> AEVAPGDVAIDGQGHVARPLTDAPGDPVEGRRLMTDRSVGNCIACHEVTEMADAQFPGTVGPSLDGVAARYPEAMIRGILVNSKNVFPETVMPAYYRVEGFNRPGIAFTSKPIE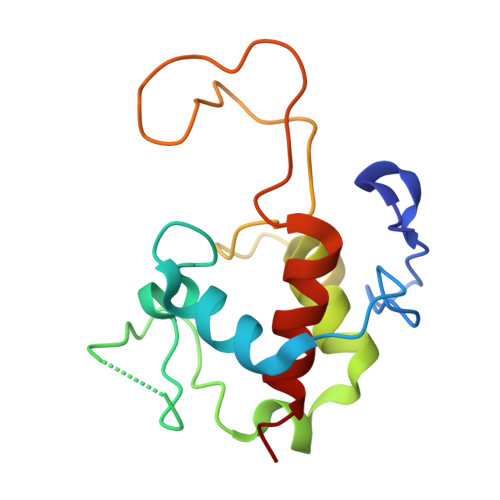GEIRPLMTAGQIEDVVAYLMTLTQ>MNNQIFESVDHYISDLLGYEDDALLAATNSLAEAGMPAISVSPNQGKFLQLLAQLCQAKNILELGTLAGYSTIWMARALPKNGRLITLEYDPKHAAVAQKNIDRAGLTSQVQIRTGKAIDILPQLVEEGAGPFDMIFIDADKPPYTEYFQWALRLSRPGTLIVADNVIRDGKVLDENSTEPAVQGARRFNAMLG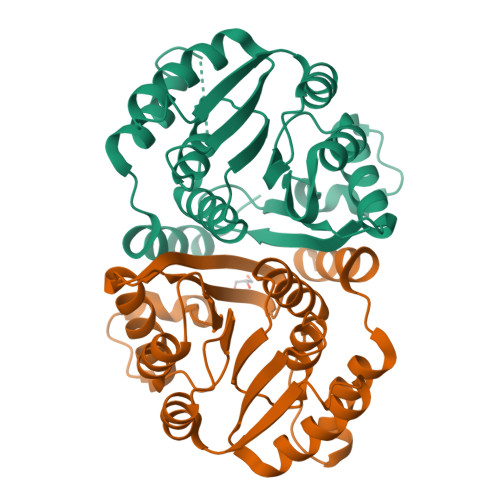ANTAVDATILQMVGVKEYDGMALAIVKLEHHHHHH[4x]> MSDNLTELSQQLHDASEKKQLTAIAALAEMGEGGQGILLDYLAKNVPLEKPVLAVGNVYQTLRNLEQETITTQLQRNYPTGIFPLQSAQGIDYLPLQEALGSQDFETADEITRDKLCELAGPGASQRQWLYFTEVEKFPALDLHTINALWWLHSNGNFGFSVQRRLWLASGKEFTKLWPKIGWKSGNVWTRWPKGFTW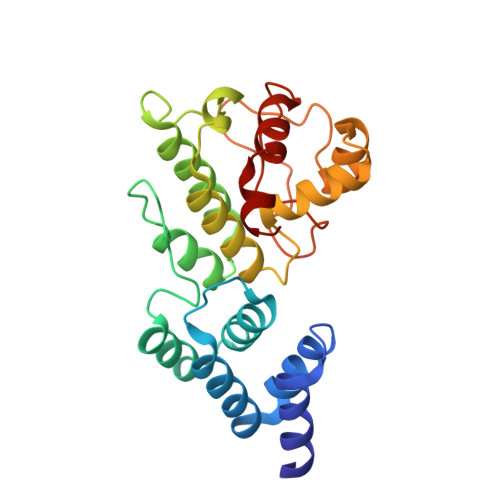DLSAPQGHLPLLNQLRGVRVAESLYRHPVWSQYGW>MGSSHHHHHHSSGLVPAGSHSKVFIRSAINRVHQNSA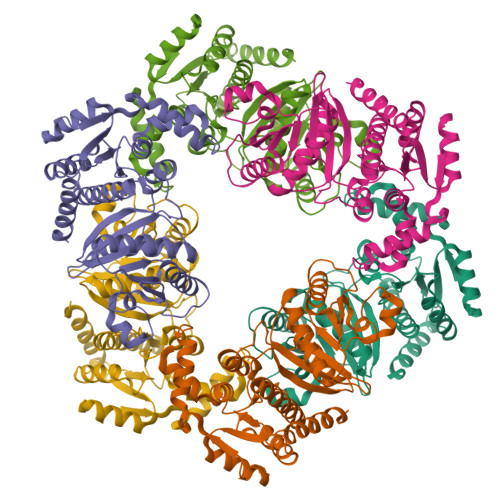ANGGELPRIVFPEGTSTKVLKALATLVEEKICQPILLGYPERVKEKIKALDIPLLNDVSIVHPSSHPKYFSFVEKLYSLEQRKGINLGEAERLMADPNYFAAMMVNQGEADGMVSGSSINYADAVRPILQTIGVYKEGIPAGLNFVLLEDKFLVLADTTVNLNPTAEQCAQIALQAAKIVEYFGIEPRVAMLSYSNFSGAEGTPRKMKKAAEIARSLRPDLMIEGDMQADTAVNPEIMERLFPFSGLKGGANVLVFPNLESSNIAYKLIQQIGKAEVIGPFLTGVRRSANVLQRTTTVDGIVNSVVFTALEAQYIKEVLKSRGKK[6x]Extensive studies have identified that many RNA-binding proteins, such as FUS, hnRNPA1, and TDP43, largely contribute to this conditional cellular compartmentation. These proteins commonly contain low complexity (LC) domains that can drive the full-length proteins to undergo liquid–liquid phase separation (LLPS) via weak multivalent interactions. In this work, we directly visualize temperature-sensitive amyloid fibrils in the liquid-like droplets of hnRNPA1 by transmission electron microscopy (TEM). Our work bridges the liquid phase and solid phase of hnRNPA1 and illuminates the functional role of reversible amyloids in the assembly of stress granules and the pathological risk as intermediates en route to irreversible fibrils.

The result showed that segment 209GFGGNDNFG217 (named hnRAC1), but not the others, formed hydrogel at 4 °C. The hydrogel was composed of amyloid fibrils observed by TEM. As temperature increased to 25 °C, the fibrils disassociated spontaneously, resembling the behavior of full-length hnRNPA1. To reveal the structural basis underlying the reversible amyloid formation of hnRAC1, we determined the atomic structure of hnRAC1 in the fibrillar form to the resolution of 1.0 Å by micro-electron diffraction (micro-ED) and to 1.4 Å by micro-focus X-ray diffraction. HnRAC1 formed needle-like crystals that diffracted both electron and X-ray beams well. The structure revealed a cross-β architecture (or steric zipper) with hydrophilic sheet interface composed by N213 and N215. Moreover, the hnRAC1 structure exhibits a distinct feature of negatively charged D214 continuously stacking along the parallel in-register β-sheets. Stacking-D engenders instability to the fibril architecture due to electrostatic repulsion and hence is barely seen in pathological fibrils. Note that in the local chemical environment of the hnRAC1 crystal, D214 is in contact with the amino terminus of hnRAC1. In contrast, as we mutated D214 to V or N, although the resulted peptides still formed amyloid fibrils with no profound structural change, unlike the WT fibril, the mutant fibrils were stable and did not dissociate as temperature increased. Similarly, in the hnRAC1 structure, kink at G211 enables the aromatic ring of F210 to reach out and interact with the Phe residues from neighboring molecules via π–π stacking.

> GFGGNDNFG>MDVTIQHPWFKRTLGPFYPSRLFDQFFGEGLFEYDLLPFLSSTISPYYRQSLFRTVLDSGISEVRSDRDKFVIFLDVKHFSPEDLTVKVQDDFVEIHGKHNERQDDHGYISREFHRRYRLPSNVDQSALSCSLSADGMLTFCGPKIQT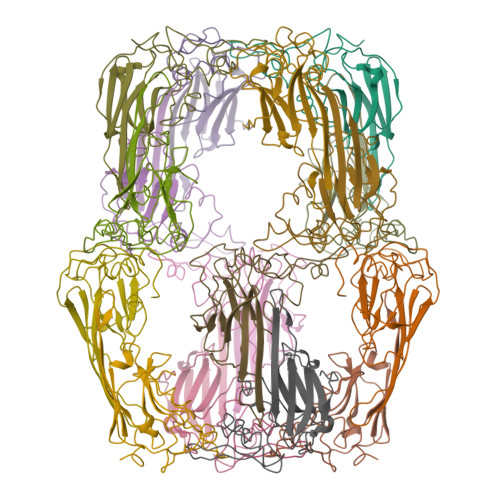GLDATHAERAIPVSREEKPTSAPSS[16x]[3,5-bis(bromanyl)-4-oxidanyl-phenyl]-(2-ethyl-1-benzofuran-3-yl)methanone | C17 H12 Br2 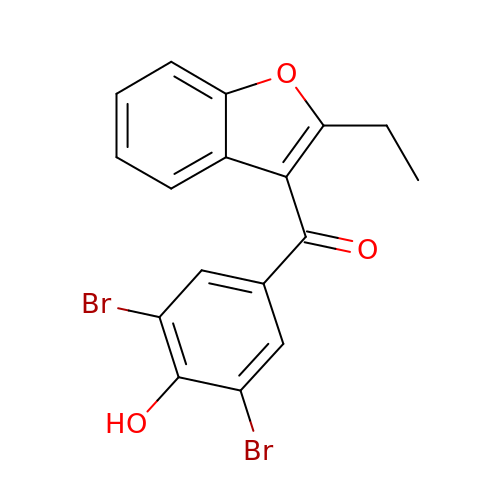O3 | WHQCHUCQKNIQEC-UHFFFAOYSA-N>MLTIGVIGKSVHPYWSQVEQGVKAAGKALGVDTKFFVPQKEDINAQLQMLESFIAEGVNGIAIAPSDPTAVIPTIKKALEMGIPVVTLDTDSPDSGRYVYIGTDNYQAGYTAGLIMKELLGGKGKVVIGTGSLTAMNSLQRIQGFKDAIKDSEIEIVDILND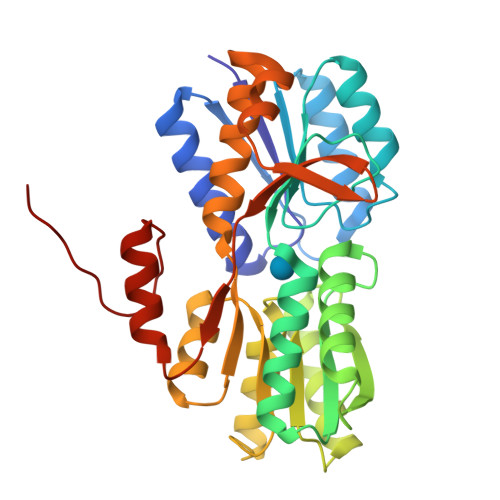EEDGARAVSLAEAALNAHPDLDAFFGVYAYNGPAQALVVKNAGKVGKVKIVCFDTTPDILQYVKEGVIQATMGQRPYMMGYLSVTVLYLMNKIGVQNTLMMLPKVKVDGKVDYVIDTGVDVVTPENLDEYLKKMEELGIPIKFGSHHHHHH[2x]> MEQSVANLVDMRDVSFTRGNRCIFDNISLTVPRGKITAIMGPSGIGKTTLLRLIGGQIAPDHGEILFDGENIPAMSRSRLYTVRKRMSMLFQSGALFTDMNVFDNVAYPLREHTQLPAPLLHSTVMMKLEAVGLRGAAKLMPSEL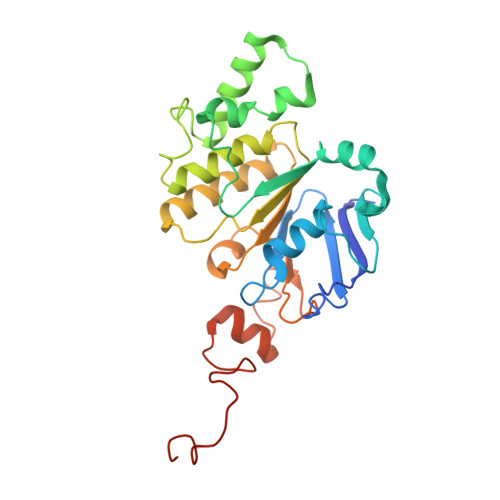SGGMARRAALARAIALEPDLIMFDQPFVGQDPITMGVLVKLISELNSALGVTCVVVSHDVPEVLSIADHAWILADKKIVAHGSAQALQANPDPRVRQFLDGIADGPVPFRYPAGDYHADLLPGS> SGRAFGEQLLKNPLIEFCDSVCRGCGQVMFQNNTVTGLLFFAGIFYNSTTLGVCAVLGTAASTLTAQLLGVDKPLVRAGLFGFNGTLAGIALPFFFNYEPAMLGYVALNGAFTTIIMASLLNFLGKWGVPALT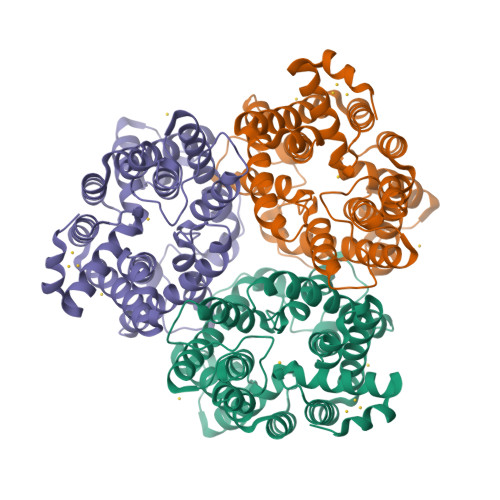APFVLATWLLMFGVYKLSLFHPGALIAPALPSVAGLADMGTVTGRTFMEGLFKGVGEVMFQDNIVTGVIFVVAILVNSRISALFAVIGSLVGLCTALIMHSPETPVRLGLYGFNSVLCGIAMGGIFFYLNIRTFLYALGCMVLGAIATGAFSVLLSPIGMPALTWPFIVVTWLFLFAGSMFRNIAQVPTEKAGTPEDNLRSLAIGSR>[3x]MGLGDPSVATVEDVSPTVFPAGPLFPTEGRIVQLFEKNTYSVVNIFDVTLRPQLKMTGVVEIPEGNGSGVVWDGQGYIVTNYHVIGNALSRNPSPGDVVGRVNILASDGVQKNFEGKLVGADRAKDLAVLKVDAPETLLKPIKVGQSNSLKVGQQCLAIGNPFGFDHTLTVGVISGLNRDIFSQTGVTIGGGIQTDAAINPGNAGGPLLDSKGNLIGINTAIFTQTGTSAGVGFAIPSSTVLKIVPQLIQFSKVLRAGINIELAPDPVANQLNVRNGALVLQVPGKSLAEKAGLHPTSRGFAGNIVLGDIIVAVDDKPVKNKAELMKILDEYSVGDKVTLKIKRGNEDLELKISLEEKSSLEHHHHHH

Plant Deg5 and Deg8 are two members of the HtrA proteases, a family of oligomeric serine endopeptidases that are involved in a variety of protein quality-control processes. These two HtrA proteases are located in the thylakoid lumen and participate in high-light stress responses by collaborating with other chloroplast proteins. Deg5 and Deg8 degrade photodamaged D1 protein of the photosystem II reaction centre, allowing its in situ replacement. The functional unit of the HtrA proteases is a trimer, with three protease domains forming a central core.

The crystallized Deg8 (S292A) contains 358 amino-acid residues (Leu91–Ser448), of which residues 104–448 could be defined in the electron-density map. The catalytic triad of Deg8 consists of His171, Asp214 and Ser292. Deg8 contains one PDZ domain that shows a different orientation compared with that in the Deg1 hexamer. As such, the Deg8 PDZ domain is flattened out from the trimeric core made by the protease domain and the concavity of the trimeric funnel is shallower than in Deg1. The Deg8 (S292A) hexamer has a narrower cavity and a distorted His171 like His147 in Deg5. Six pairs of hydrogen bonds are observed between Arg179 and Phe389* from opposite trimers, stabilizing the hexamer. Trimerization is primarily mediated by hydrophobic interactions and hydrogen bonds. The recombinant Deg8 exhibits a remarkably lower proteolytic activity than that of Deg1 in degrading substrate. This incompetent state suggests that to activate Deg8 a new activation mechanism may be employed for rearrangement of the activation domain.>[2x]RIVEIPVCYGGEFGPDLEEVAKINQLSPEEVIDIHTNGEYVVYMLGFAPGFPFLGGMSKRIAAPRKSSPRP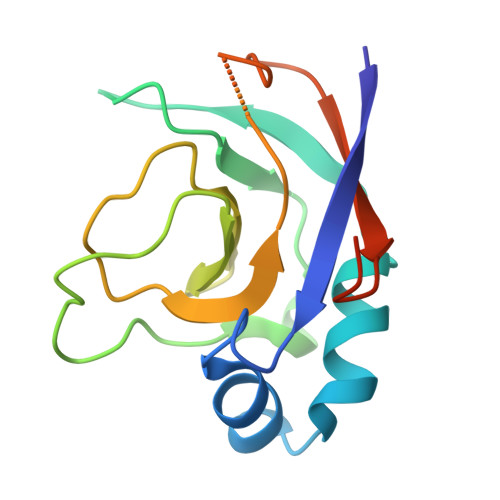SIPAGSVGIAGLQTGVYPISTPGGWQLIGKTPLALFRPQENPPTLLRAGDIVKFVRISEKDYHAYKEESN>[4x]MEGTGVVAVYGNGAITEAKKSPFSVKVGLAQMLRGGVIMDVVNAEQARIAEEAGACAVMALERVPADIRAQGGVARMSDPQMIKEIKQAVTIPVMAKARIGHFVEAQILEAIGIDYIDESEVLTLADEDH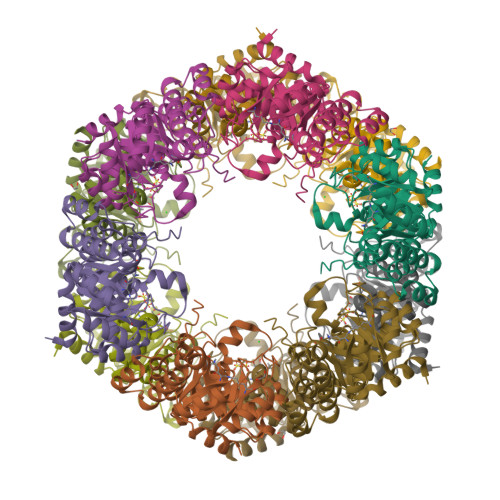HINKHNFRIPFVCGCRNLGEALRRIREGAAMIRTKGEAGTGNIIEAVRHVRSVNGDIRVLRNMDDDEVFTFAKKLAAPYDLVMQTKQLGRLPVVQFAAGGVATPADAALMMQLGCDGVFVGSGIFKSGDPARRARAIVQAVTHYSDPEMLVEVSCGLGEAMVGINLNDEKVERFANRSEHHHHHH> ENTISFFDSGDPERMNNEALMRGCGEQIVNLRPLLRTFRTINDNWSLAANTKTP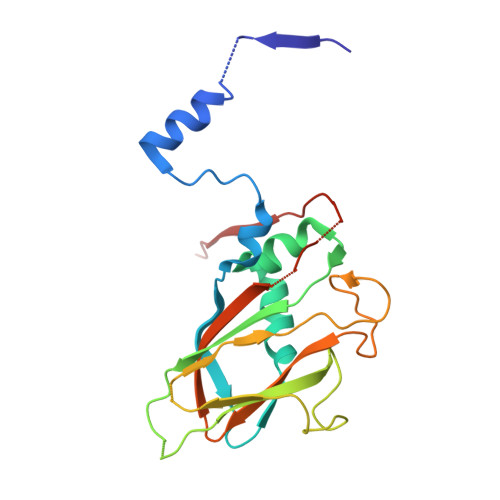ITDLTNTADAEGRDYMSYLSFLYRFYRGGRRYKFFNTTPLKQSQTCYVRSFLIPRNYTADEINTDGPSHITYPVINPVHEVEVPFYSQYRKIPIASTSDKGYDSSLMYYTNVGTQQIVARAGNDDFTFGWMIGTPQLQGITKEV> MRHISPEELIALHDANISRYGGLPGMSDPGRAEAIIGRVQARVAYEEITDLFEVSATYLVATARGHISNDANKRTALNSALLFLRRNGVQVFD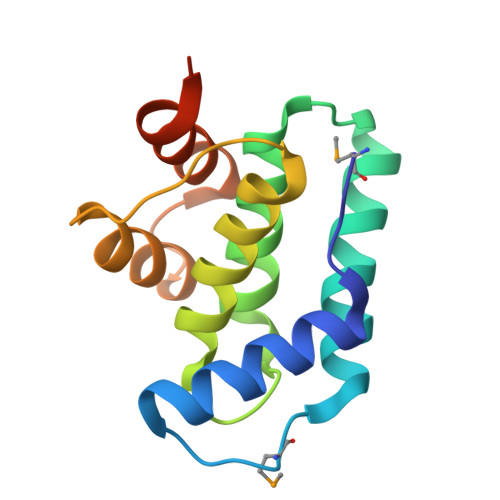SPELADLTVGAATGEISVSSVADTLRRLYGSAELEHHHHHH>[8x]HHHHHHMSSPAQPAVPAPLADLKIQHTKIFINNEWHNSVSGKKFPVLNPATEEVICHVEEGDKADVDKAVKAARQAFQIGSPWRTMDASERGRLLNKLADLMERDRLLLATMEALNGGKVFANAYLSDLGGCIKALKYCAGWADKIHGQTIPSDGDIFTYTRREPIGVCGQIIPWNFPMLMFIWKIGPALSCGNTVVVKPAEQTPLTALHLASLIKEAGFPPGVVNIVPGYGPTAGAAISSHMDVDKVAFTGSTQVGKLIKEAAGKSNLKRVTLELGGKSPCIVFADADLDIAVEFAHHGVFYHQGQCCVAASRIFVEESVYDEFVKRSVERAKKYVLGNPLTPGINQGPQIDKEQHDKILDLIESGKKEGAKLECGGGRWGNKGFFVQPTVFSNVTDEMRIAKEEIFGPVQQIMKFKSVDDVIKRANNTTYGLAAGLFTKDLDKAITVSSALQAGVVWVNCYMMLSAQCPFGGFKMS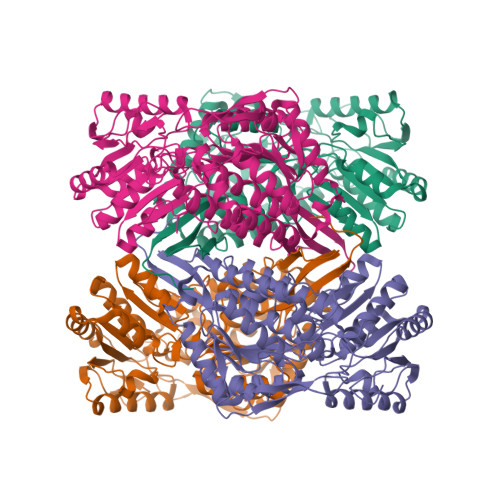GNGRELGEHGLYEYTELKTVAMKISQKNS>[2x]MGKIFEDNSLTIGHTPLVRLNRIGNGRILAKVESRNPSFSVKCRIGANMIWDAEKRGVLKPGVELVEPTSGNTGIALAYVAAARGYKLTLTMPETMSIERRKLLKALGANLVLTEGAKGMKGAIQKAEEIVASNPEKYLLLQQFSNPANPEIHEKTTGPEIWEDTDGQVDVFIAGVGTGGTLTGVSRYIKGTKGKTDLISVAVEP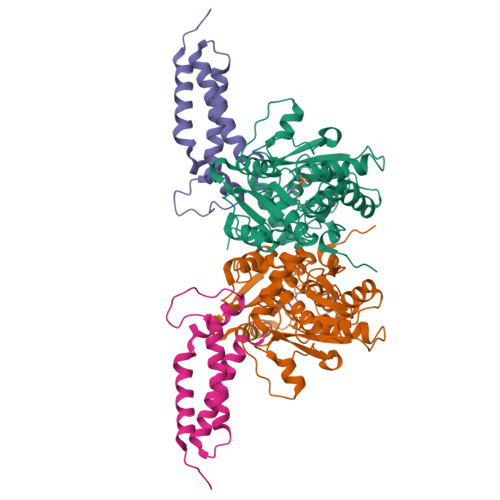TDSPVIAQALAGEEIKPGPHKIQGIGAGFIPANLDLKLVDKVIGITNEEAISTARRLMEEEGILAGISSGAAVAAALKLQEDESFTNKNIVVILPSSGERYLSTALFADLFTEKELQQ;>[2x]MAKSHHHHHHTSVENNALSLVARGCAVAAPCRTKVAEQLLEIGAKAGMAGLAGAAVKDMADRMTSDELEHLITLQMMGNDEITTKYLSSLHDKYGSGAASNPNIGKDLTDAEKVELGGSGSGTGTPPPSENDPKQQNEKTVDKLNQKQESAIKKIDNTIKNALKDHDIIGTLKDMDGKPVPKENGGYWDAMQEMQNTLRGLRNHADTLKNVNNPEAQAAYGRATDAINKIESALKGYGI FdlA from Flavobacterium sp. SA-0082 is an endo-type fucoidan-degrading enzyme that cleaves the sulfated fuco-glucuronomannan (SFGM) through a lytic mechanism. We show that the FdlA-NTD adopts a right-handed parallel β-helix fold, and possesses a substrate binding site composed of a long groove and a unique alkaline pocket. Our structural, biochemical, and enzymological analyses strongly suggest that FdlA-NTD utilizes catalytic residues different from other β-helix polysaccharide lyases, potentially representing a novel polysaccharide lyase family. Here, we report crystal structures and enzymological characterization of wild type (WT) and eight single mutants of the catalytic N-terminal domain (NTD) of FdlA, revealing its unique substrate binding pocket and identifying the key catalytic residues.

We first measured the enzymatic activity of 12 mutants and found that eight of them (D137A, K141A, H176A, F179A, E236A, R240A, Y242A, and Y242F) almost completely abolished their activities, H279A mutant retained approximately 65% of the activity compared with WT, while mutations of Asn243, Arg272, and Tyr322 to Ala only negligibly affect their activities. Mutation of Y242A resulted in a large structural change at the potential active site, with a 3 Å shift of Asn243, which narrows the substrate groove in the mutant structure. In addition, both glycosidic O atoms between −1 and +1 subsites and the carboxyl group at +1 subsite are hydrogen bonded with Tyr242, implying the essential role of Tyr242 for FdlA-NTD catalysis. Tyr242 in the substrate binding groove is located at the edge of the alkaline pocket. This arrangement, together with our observation that the pocket is able to accommodate a trisaccharide unit, strongly suggests that Tyr242 directly participates in cleaving the substrate to produce trisaccharides, and the alkaline pocket assists in orientating the polysaccharide substrate into a position close to Tyr242. Furthermore, we found that the inactive mutants failed to exhibit significant structural changes compared with the wild type, which is consistent with our CD results.

>HHHHHHSSGLVPRGSHMQTTTVYSLEDLLPYLKQDNVDVKLAPGTYNVNGFDVGEDRLFSTTPLFLFEGSNSTYDFTDVKLNINTVVLTKFGNNEVNEIQILGNNNVLKNLKLEDIGTTAPSNRAQSIVIDGRDNRIEGFHLTIRGSYPYGYGDAFGKGGGSVINHRKHSGVLIRGLRNHLKDCTIISRSYGHIVFMQAASYPTVEGCYIEGEMRSTDDMLAEEGTGSPADKVDFMTVWGYKLPAGYMMSLQEGGIRAANAGTTYIDGVEIQRATDNPTVLNCTIKNARTGVTLAHANGTKYVEGCTVLGCENGYSIGSGTVVNCGADAIYGPVFKNTYGSDKGYNADITILPPSDAYYNGHDAVAYIGGSNHNLTFRSEITEIPSNLKIMVSGDLQGLRVLHGSNPSQNNFAGTNIVLRNLTNFPVDLHSDSSNITVTSCDTDNITDNGTNNSIEAID[2x]>[4x]MSLVNTIGFDREKYIEMQSQHIRERREALGGKLYLEMGGKLFDDMHASRVLPGFTPDNKIAMLDRIKDEVEILVCINAKDLERHKIRADLGISYEEDVLRLVDVFRDRGFLVEHVVLTQLENDNRLALA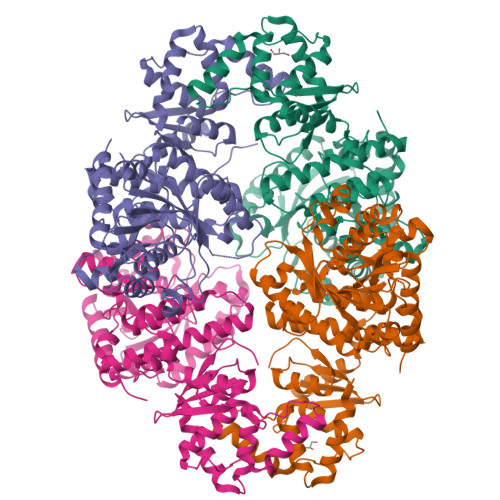FIERLQRLGIKVSRHRVIPGYPTDMDRIVSDEGFGLNEYAETTRDLVVVTAPGPGSGKLATCLSQVYHEHKRGVAAGYAKFETFPIWNLPLEHPVNLAYEAATVDLNDANVIDHFHLAAYGEQTVNYNRDVEAFPLLKTLLERLMGESPYQSPTDMGVNMAGNCISDDAACRHASEQEIIRRYFKALVEEARTGKDSTQSDRAAVVMAKAGIKASQRVVVEPARQVEERTSLPGCAIELVDGSIITGATSDLLGCSSSMLLNALKHLAGIDDAIHLLSPESIEPIQTLKTVHLGSSNPRLHTDEVLIALSVSAATDSNAQKALDQLKNLRGCDVHTTTILGSVDEGIFRNLGVLVTSDPKFQKNKLYQKREGHHHHHH We have discovered a new cluster of genes that is found exclusively in the Actinobacteria phylum. This locus includes genes for the 2-aminophenol meta-cleavage pathway and the shell proteins of a bacterial microcompartment (BMC) and has been named aromatics (ARO) for its putative role in the breakdown of aromatic compounds. In contrast, the 2-AP ring cleavage is catalyzed by 2-AP 1,6-dioxygenase (AmnAB), which oxidizes substrates with an amino group adjacent to a hydroxyl group. First, based on the co-occurence of a putative 2-AP 1,6-dioxygenase, which is suggested to catalyze the benzene ring cleavage of 2-AP (herein referred to as ARO dioxygenase), with shell proteins, the ARO BMC is the first metabolosome predicted to be involved in the degradation of aromatic substrates. Our results show the ability of recombinant ARO dioxygenase to interact with either catechol or 2-AP substrates and convert them into aldehyde intermediates, which are then detoxified by the ARO AldDh.

To structurally and functionally characterize the ARO dioxygenase and to demonstrate its ability to degrade 2-AP, we recombinantly co-expressed and purified the alpha and a His-tagged beta subunit (ARO AmnA and AmnB) from Micromonospora rosaria. The co-elution of the subunits and the observation that neither of the subunits was soluble when expressed on their own, suggest a requirement for an interaction between the two subunits during folding. This interaction was verified by size exclusion chromatography analysis, which yielded a major peak at 140 kDa, corresponding to a tetramer composed of two heterodimers, as observed for other dioxygenases. We determined the crystal structure of the ARO dioxygenase from Micromonospora rosaria at 1.75 Å resolution. Two alpha/beta heterodimers form a biological dimer via their beta subunits, consistent with our size exclusion analysis, and we find two of those in the asymmetric unit of the P1 unit cell. We can model residues D3 to H278 of the alpha subunit and T30 to G322 of the beta subunit, as well as the iron atom in the active site into the electron density. The lack of density for the first 29 amino acids for the beta subunit is consistent with the possibility that this extension is involved in encapsulation; in structures of BMC-associated enzymes with EPs, the extensions are typically not visible in the electron density, as exemplified in the crystal structures of both PDU1C-associated flavodoxin and the GRM3-associated AldDh. However, one large difference between the ARO BMC-associated dioxygenase and its non-BMC-associated counterpart is in a loop close to the active site for the beta subunit involving residues N184-Y188 (orange). A consequence of the difference is a much more shielded active site as seen in the surface representation.

>[4x]MADRTGIVAGALLPGMPHLLAEHPAPSWSALAGAARDVGARLRRLEPDVVLLLSTQWFTVLGHQFQCDPNPRGEHVDENWYAYDYGLLDYDLRFDVDFTERWADRVQAGGMQARRTRYDGFPIDTGTIVTSALLDPDRRLRWAQVSCNLYADADTLADVGRAGAAAARDAGLRAAVVVVTGMSSGLIQQWIEPGQDRIGEPGHDQWNTRVLDLLTAGKVDEVLAVREDFARQAQADSQFRALAFAAGAEATTGPAHLHAYGPIWGTGAAVLSWNLPDHP;>[4x]MSRVFRVPLAPTRGGATTAPRTPAPAPAPTRPGIVAGCLSPHPPHLIYGENPPQNEPRSTGGWETLRWAYERLRARIRDVHKPDVLIVHAPHWITMVGHHVNCVPNPRGLSVEPIFPHLFRYRYDFRTDVELGEAIAEEASGLGLVTRTLRDPRVRVDYATIGALHLANPAWDIPVVSLSANNNPYFYSDASLTEMEVLGEATRLAVEATGRRAVLLASNSLSHLHWHEEPELPEDMEREHPYNNHQYRWDMKLLEAIRRGPTAPLRDLIPEHIEATASETKAGSLTWMLAAMGWPKVAGDVLGYGTIIGTGNAIVEWLPEGSHHGGSGGSHHHHHH> MSASQSAVRSRAEAV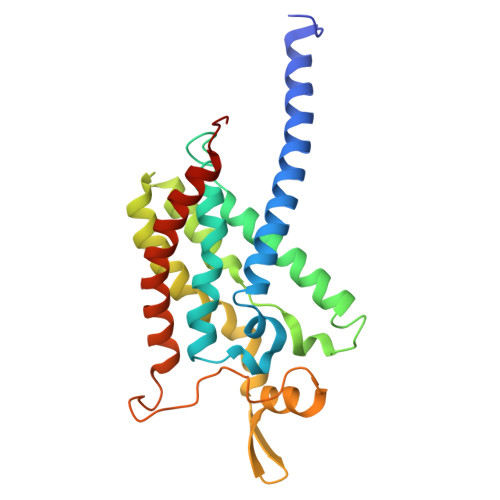KVSRTFDYMILFTVFFVVLGGYHIHYMLTGGDWDFWTDWKDRRLWVTVAPIVSITFPAAVQAVLWWRYRIAWGATLCVLGLLLGEWINRYFNFWGWTYFPVNFVFPSNLMPGAIVLDVILMLSNSMTLTAVVGGLAWGLLFYPGNWPIIAPLHVPVEYNGMMMTLADLQGYHYVRTGTPEYIRMVEKGTLRTFGKDVAPVSAFFSGFVSILIYFLWHFFGSWFGSEKFVQAA> AADFDFLKNLSLEELQMRLKALDPMM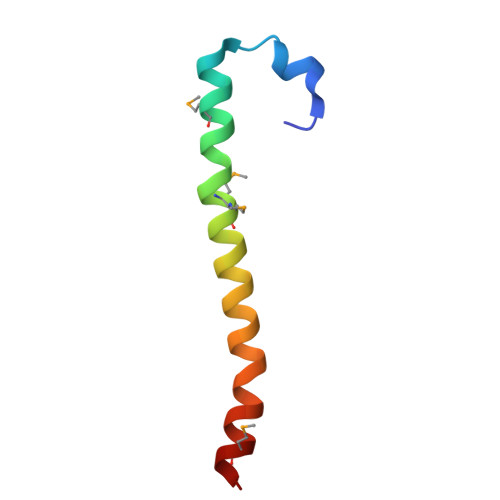EREIEELRQRYTAKRQPILDAMDAK>[6x]ATSMSFVIWITG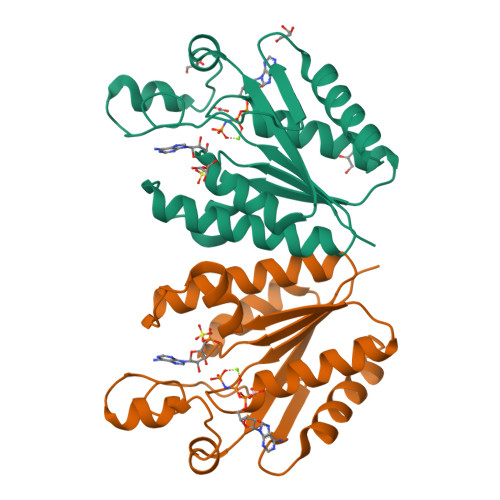PSGAGKTTLANALYKKLESMGYRVELLDGDGVRRKLYPNLGFSEEERWMHNRVVVEMARRLSRNGIITIVSVVSPYRAWREYARKEIEKFVEVYPRCPLEVRMKRDPKGLYSKALRGEIKGLTGLDGEYEEPENPEVVVDTDKMTVEEEVEAVLKKLMELGYL> MKHHHHHHMKQNSPLDEENLTQENQDRGTHVDRGLASANVDFAFSLYKQLVLKAPDKNVIFSPLSISTALAFLSLGAHNTTLTEILKGLKFNLTETSEAEIHQSFQHLLRTLNQSSDELQLSMGNAMFVKEQLSLLDRFTEDAKRLYGSEAFATDFQDSAAAKKLINDYVKNGTRGKITDLIKDLDSQTMMVLVNYIFFKAKWEMPFDPQDTHQSRFYLSKKKWVMVPMMSLHHLTIPYFRDEELSCTVVQLNYTGNASALFILPDQDKMEEVEAMLSRETLARWGDSLEFREIGELYLPKFSISRDYNLNDILLQLGIEEAFTSKADLSGITGARNLAVSQV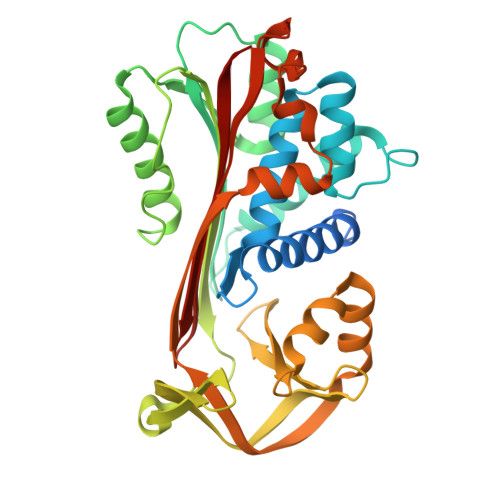VHKAVLDVFEEGTEASAATAVKITLL>[2x]MEHSVIHSTFTIERTYPQSPDRVFHAFADKATVRRWRVDGDGFTVAEFSFDFRVGGGEVSRFSYGGGPEVRLDAQFQDIVPDQRIVFSYRMAIGPQPMSASLTTVELTPSGDGT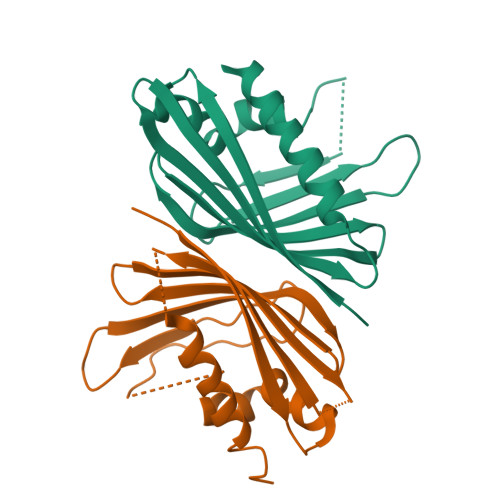RLTYTEQGAFFDGVDSAKGREEGTRGLLEALAAELQKWKLEHHHHHH> VTGDTDQPIHIESDQQSLDMQGNVVTFTGNVIVTQGTIKINADKVVVTRPGGEQGKEVIDGYGKPATFYQMQDNGKPVEGHA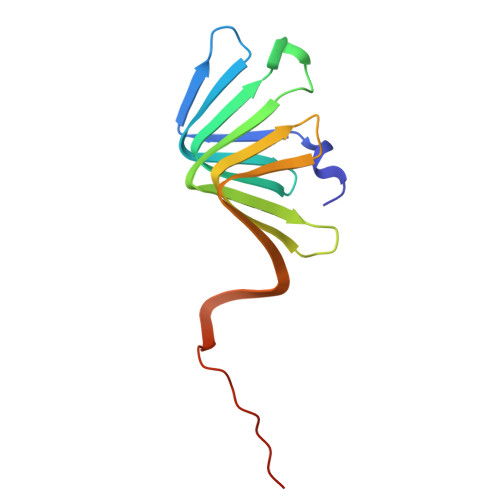SQMHYELAKDFVVLTGNAYLQQVDSNIKGDKITYLVKEQKMQAFSDKGKR> GRRQLPCAKALYNYEGKEPGDLKFSKGDIIILRRQVDENW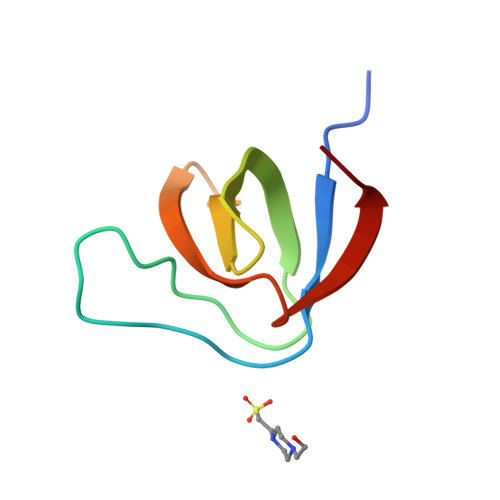YHGEVNGIHGFFPTNFVQIIKPL>[5x]GMQTKVINFNDKFSLFNQHWSPRV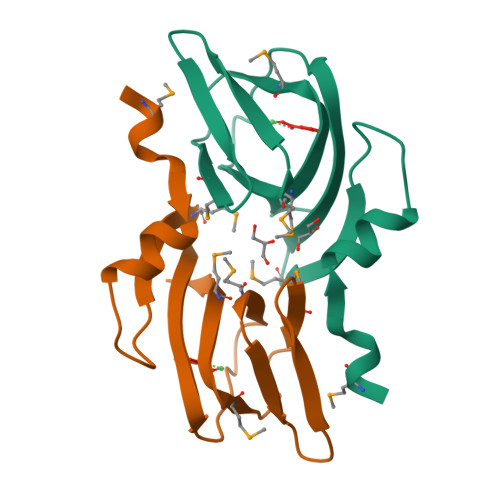IAEMNDYQFKLVKVEGEFVWHEHADTDEVFIVMEGTLQIAFRDQNITLQAGEMYVIPKGVEHKPMAKEECKIMIIEPR(2E)-3-(4-hydroxyphenyl)-1-(2,4,6-trihydroxyphenyl)prop-2-en-1-one | C15 H12 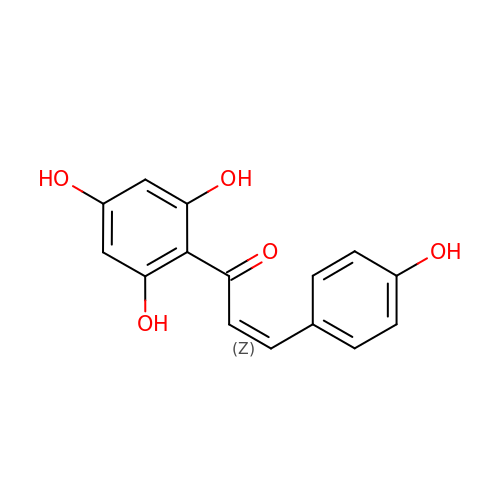O5 | YQHMWTPYORBCMF-UHFFFAOYSA-N>TPEMPVLENRAAQGNITAPGGARRLTGDQTAALRNSLSDKPAKNIILLIGDGMGDSEITAARNYAEGAGGFFKGIDALPLTGQYTHYALNKKTGKPDYVTDSAASATAWSTGVKTYNGALGVDIHEKDHPTILEMAKAAGLATGNVSTAELQDATPAALVAHVTSRKCYGPSATSQKCPGNALEKGGKGSITEQLLNARADVTLGGGAKTFAETATAGEWQGKTLREEAEARGYQLVSDAASLNSVTEANQQKPLLGLFADGNMPVRWLGPKATYHGNIDKPAVTCTPNPQRNDSVPTLAQMTDKAIELLSKNEKGFFLQVEGASIDKQNHAANPCGQIGETVDLDEAVQRALEFAKKEGNTLVIVTADHAHASQIVAPDTKAPG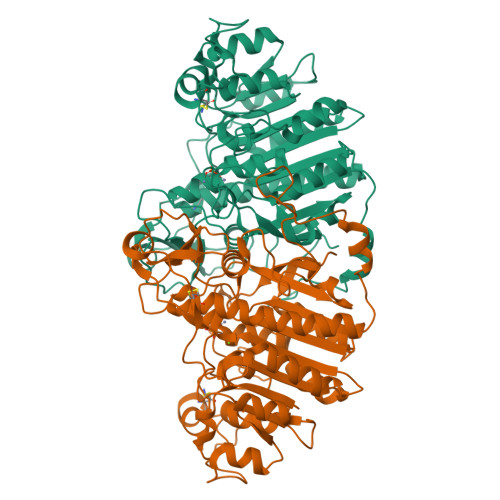LTQALNTKDGAVMVMSYGNSEEDSQEHTGSQLRIAAYGPHAANVVGLTDQTDLFYTMKAALGLK[2x]> HMLEAKFEEASLFKRIIDGFKDCVQLVNFQCKEDGIIAQAVDDSRVLLVSLEIGVEAFQEYRCDHPVTLGMDLTSLSKILRCGNNTDTLTLIADNTPD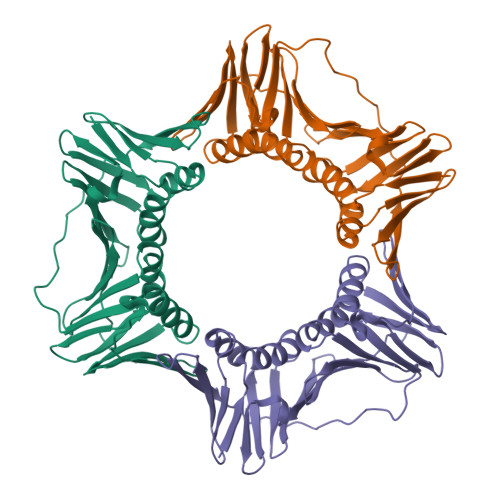SIILLFEDTKKDRIAEYSLKLMDIDADFLKIEELQYDSTLSLPSSEFSKIVRDLSQLSDSINIMITKETIKFVADGDIGSGTVIIKPFVDMEHPETSIKLEMDQPVDLTFGAKYLLDIIKGSSLSDRVGIRLSSEAPALFQFDLKSGFLQFFLAPKFNDEE>MKSTSDLFNEIIPLGRLIHMVNQKKDRLLNEYLSPLDITAAQFKVLSSIRSAASITPVELKKVLSVDLGALTRMLDRLVCKGW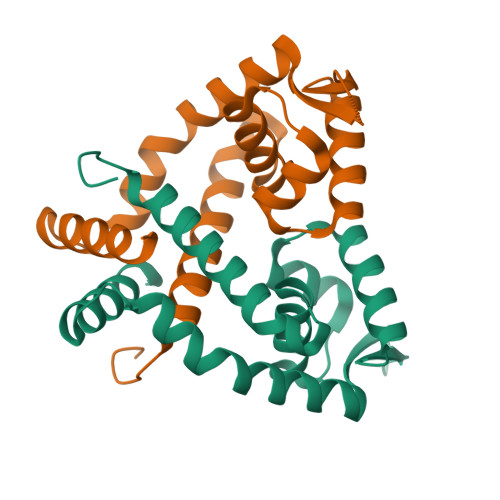VERLPNPNDKRGVLVKLTTGGAAISEQSHQLVGQDLHQELTKNLTADEVATLEYLLKKVLP[2x]>[2x]SNAEERRVAYPVLRELTERTGETSALMVWNGNESMCVEQIPSRHQVKHLAPLGARYNEALSSSVQVFLASENEDRVRQLLRSGSITLTGVD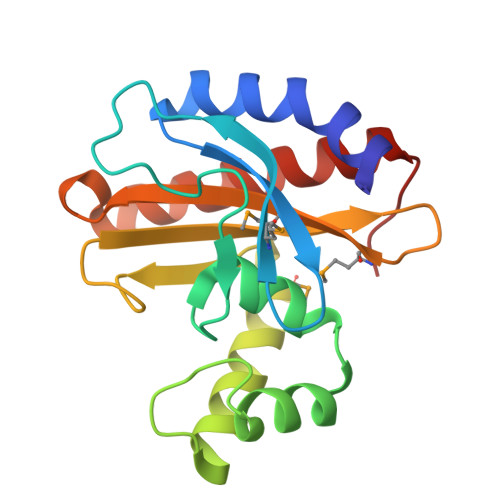EDAVEAYLLRLKESMERGWAVNFGETSIEEVGVASPVYDHRGNMVASVLIPAPKFRVSQDTLNSLGEACAAAAAKVTTRLGGRAP1-(5-O-phosphono-beta-D-ribofuranosyl)-N-(4-{[3-(trifluoromethyl)phenyl]sulfonyl}benzyl)-1H-pyrazolo[3,4-b]pyridine-5-carboxamide | C26 H24 F3 N4 O10 P S | 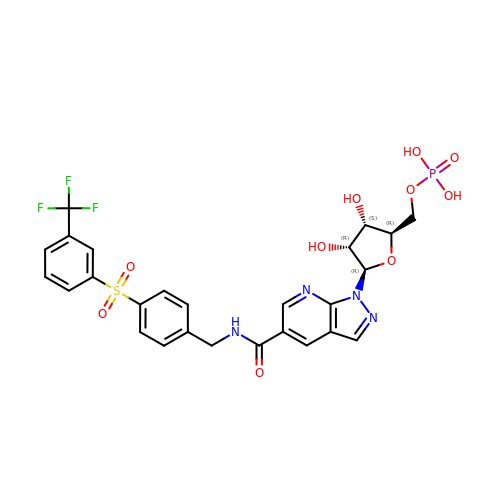MBKCNGJHWVWHDL-NMOFPLQQSA-N As a proof of concept, we used this platform to identify both known and novel L- and D-amino acid peptide binders to the well-characterized model target, streptavidin. All peptides bind within or near the biotin binding pocket of streptavidin formed by two surface loops [1/2 (amino acids 22–28) and 3/4 (amino acids 42–52)], and by antiparallel β-sheets involved in an extensive polar interaction network, in which residues Ser88 and Thr90 of β-strand 6 play a major role. The surface loops of streptavidin are flexible: upon biotin binding they undergo a conformational change to form a closed conformation, but to accommodate the peptide ligands, loop 3/4 is dislocated by 13–16 Å from the biotin closed form to adopt a well-defined peptide-specific structure. All eight L- and D-peptides discovered in this work bind to the same pocket of streptavidin in distinctive binding modes suggesting (1) the rich malleability of L- and D-peptides and (2) the ability of streptavidin itself to adjust the flexible loop to accommodate multiple peptides with diverse sequences and conformations.

The peptides FDEWL, LAEYH, and PAWAH were selected as representative sequences from distinct clusters, along with the abundant HPQ motif, as hotspot sequences for the next step of evolution. Instead, Asn2 forms a hydrogen bond with Ser45; the backbone NH of the C-terminal Gly12 forms a hydrogen bond with Asn85. The negatively charged sidechain of Asp5 forms a salt-bridge with Arg84 and contributes to a network of polar interactions with Ser52 and Ser45. Further, Phe4, Trp7, and Leu8 are involved in critical van der Waals interactions with Trp79 and Trp120 from a neighboring streptavidin subunit [Fig. 5(A)]. For example, the substitution plot reveals a clear preference for Asp over Glu at position 5, which can be explained by the multiple polar interactions that the short Asp5 sidechain—but not the longer Glu sidechain—can accommodate. Because GNSFDDWLASKG forms an α-helix, a repeating pattern of conserved residues alternates with non-conserved positions in steps of 2–3 amino acids. With the exception of these flexible loops, streptavidin has a rigid structure, with a root mean square deviation (rmsd) of ~0.5 Å for a superposition of all atoms in the co-crystal structures. The Gdlwqheatwkkq, GGwhdeatwkpG and GNSFDDWLASKG peptides bind with the same N-terminus to C-terminus directionality, opposite to the binding orientation of all other peptides. As the array data would predict, the linear version, NH2-NQpWQ-COOH, exhibited no measurable binding at peptide concentrations of ≤2 mM. The GNSFDDWLASKG L-peptide demonstrated irreversible binding kinetics, making it impossible to determine a Kd value [Supplementary Fig. 4(C)].

>[8x]MRKIVVAAIAVSLTTVSITASASADPSKDSKAQVSAAEAGITGTWYNQLGSTFIVTAGADGALTGTYESAVGNAESRYVLTGRYDSAPATDGSGTALGWTVAWKNNYRNAHSATTWSGQYVGGAEARINTQWLLTSGTTEANAWKSTLVGHDTFTKVKPSAASIDAAKKAGVNNGNPLDAVQQ;>[8x]GNSFDDWLASKGX> GSHMTEKVLQICPKDMRADICVHLNRKVFK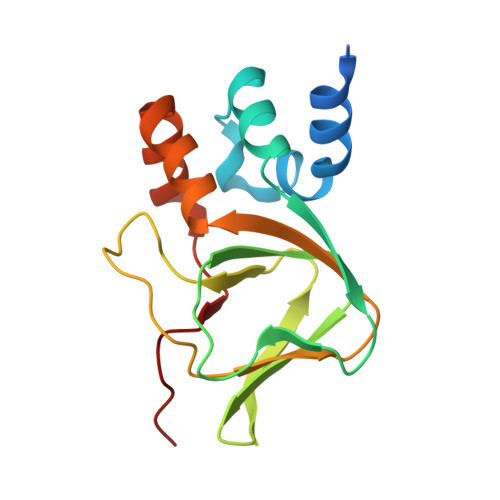EHPAFRLASDGCLRALAMEFQTVHCAPGDLIYHAGESVDSLCFVVSGSLEVIQDDEVVAILGKGDVFGDVFWKEATLAQSCANVRALTYCDLHVIKRDALQKVLEFYTAFSHSFSRNLILTYNLRKRIVF>MSFELPALPFAKDALEPHISAETLDYHHGKHHNTYVVKLNGLIPGTEFEGKTLEEIIKTSTGGVFNNAAQIWNHTFYWNCLAPNAGGQPTGAVAAAIDAAFGSFEEFK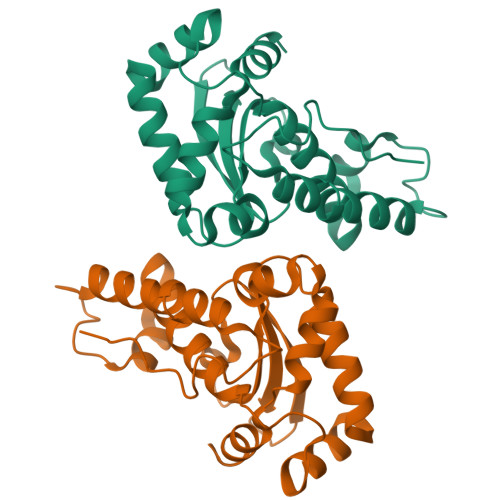AKFTDSAINNFGSSWTWLVKNADGSLAIVNTSNAATPLTDEGVTPLLTVDLWEHAYYIDFRNVRPDYMGAFWSLVNWSFVEENLAK[2x]>MLLSDRDLRAEISSGRLGIDPFDDTLVQPSSIDVRLDCLFRVFNNTRYTHIDPAKQQDELTSLVQPVDGEPFVLHPGEFVLGSTLELFTLPDN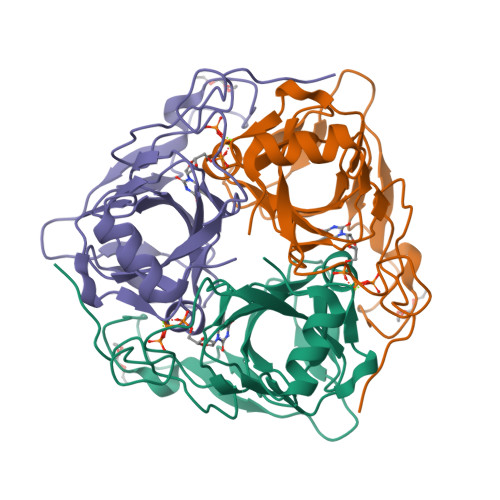LAGRLEGKSSLGRLGLLTHSTAGFIDPGFSGHITLELSNVANLPITLWPGMKIGQLCMLRLTSPSEHPYGSSRAGSKYQGQRGPTPSRSYQNFIRST[2x]(1R)-3-(3,4-dimethoxyphenyl)-1-{3-[2-(morpholin-4-yl)ethoxy]phenyl}propyl 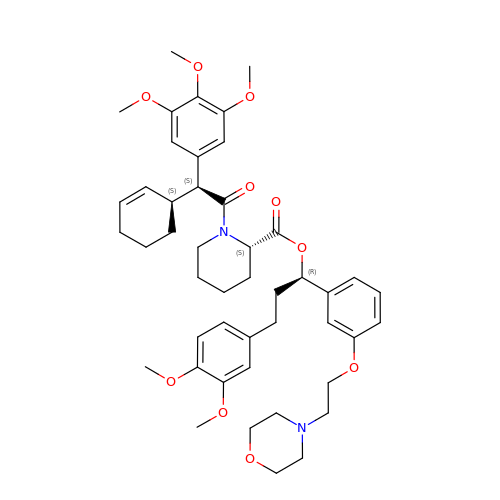(2S)-1-[(2S)-2-[(1S)-cyclohex-2-en-1-yl]-2-(3,4,5-trimethoxyphenyl)acetyl]piperidine-2-carboxylate | C46 H60 N2 O10 | LMMQNDBBWIKJQS-CNKHDIINSA-N>[12x]SLKEKIEKLVEELIRHTEELRELLEKLVKHGGASEEYLLELLENLVRLAHVIAEVAREQGNEELLEEA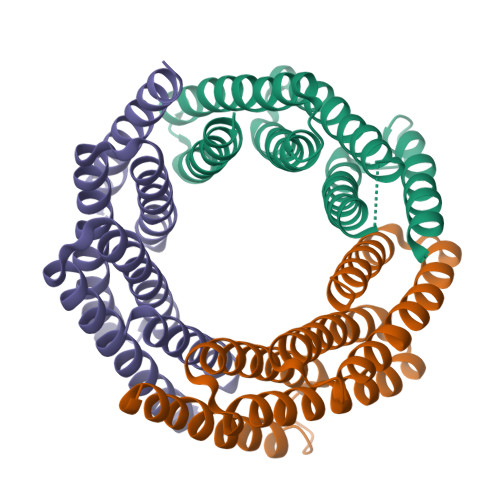ARLAEEAARQAEELAREARREGNLELALKALQILVNAAYVLAEIARDRGNEELLEKAERLAREALRQVREISKRLQKEGNIELALKANRLLIDALRVLVRIMRHR Biogenesis of the large ribosomal (60S) subunit involves the assembly of three rRNAs and 46 proteins, a process requiring approximately 70 ribosome biogenesis factors (RBFs) that bind and release the pre-60S at specific steps along the assembly pathway. The methyltransferase Spb1 and the K-loop GTPase Nog2 are essential RBFs that engage the rRNA A-loop during sequential steps in 60S maturation. Spb1 methylates the A-loop nucleotide G2922 and a catalytically deficient mutant strain (spb1D52A) has a severe 60S biogenesis defect. Nog2 is an essential hub enzyme that acts as a key quality control element during the nucleoplasmic maturation of 60S, anchoring both the pre- and post-rotation states of the 5S rRNP (Nog2pre and Nog2post) via extensive rRNA and RBF interactions.

Refinement of the Rix1-containing subset to 2.9 Å resolution shows that GDP-bound Nog2 remains associated with the 60S during 5S rotation and Rix1 complex binding, as the Nog2 active site in this reconstruction also contains GDP and lacks clear density for the A-loop. Just like Nog2pre, Nog2post is not destabilized by the presence of Nog2-GDP, indicating that 5S rotation, Rix1-complex binding and Rea1 recruitment can proceed normally in the context of Nog2-GDP. Because the presence of Nog2-GDP did not cause any structural defects or instabilities in late nucleoplasmic intermediates, we instead hypothesized that the 60S biogenesis defect of the spb1D52A strain arises during the nucleolar/nucleoplasmic transition of pre-60S particles. Our finding that the spb1D52A suppressor mutations sustain near wild-type growth even though Nog2 is GDP-bound throughout the nucleoplasmic maturation of the large subunit shows that although hydrolysis is necessary for Nog2 release, these events can be uncoupled without affecting the timing of Nog2 release and Nmd3 binding. This suggests that at a specific point in late nucleoplasmic maturation, after Rix1-Rea1 mediated removal of Rsa4, Nog2 binding to the pre-60S depends on the presence of the GTP γ-phosphate.

> MGTGKKEKSRRIREGDTKDGNLRVKGENFYRDSKRVKFLNMYTSGKEIRNKKGNLIRAASFQDSTIPDARVQPDRRWFGNTRVISQDALQHFRSALGETQKDTYQVLLRRNKLPMSLLEEKDADESPKARILDTESYADAFGPKAQRKRPRLAASNLEDLVKATNEDITKYEEKQVLDATLGLMGNQEDKENGWTSAAKEAIFSKGQSKRIWNELYKVIDSSDVVIHVLDARDPLGTRCKSVEEYMKKETPHKHLIYVLNKCDLVPTWVAAAWVKHLSKERPTLAFHASITNSFGKGSLIQLLRQFSQLHTDRKQISVGFIGYPNTGKSSIINTLRKKKVCQVAPIPGETKVWQYITLMKRIFLIDCPGIVPPSSKDSEEDILFRGVVRVEHVTHPEQYIPGVLKRCQVKHLERTYEISGWKDATEFIEILARKQGRLLKGGEPDESGVSKQILNDFNRGKIPWFVLPPEKEGEEKPKKKEVEKTA>MFFTTPQPELSFDAMTIVGNLNKTNAKKLSDFMSTEPQIRLWDILQTKFKAKALQEKVY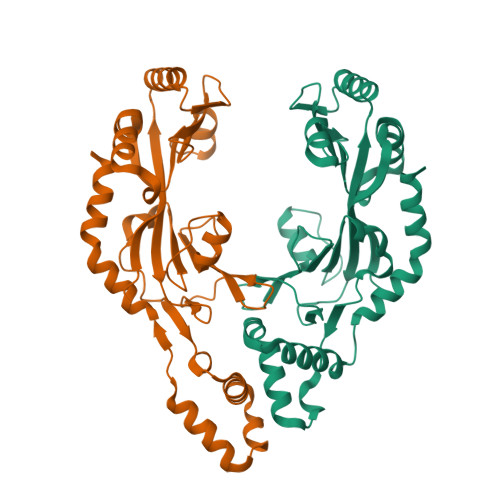IEYDKVKADSWDRRNMRVEFNPNKLTHEEMLWLKQNIIDYMEDDGFTRLDLAFDFEDDLSDYYAMTDKAVKKTIFYGRNGKPETKYFGVRDSDRFIRIYNKKQERKDNADVEVMSEHLWRVEIELKRDMVDYWNDCFNDLHILQPDWKTIERTSDRAMVFMLLNDEEEWGKLERRTKNKYKKLIKEISLIDLTDLMKSTLKANEKQLQKQIDFWQREFRFWK[2x]> ALWQFNGMIKCKIPSSEPLLDFNNYGCYCGLGGSGTPVDDLDRCCQTHKNCYKQAKKLDSCKVLVDNPYTNNYSYSCSNNEITCSSENNACEAFICNCDRNAAICFSKVPYNKEHKNLDK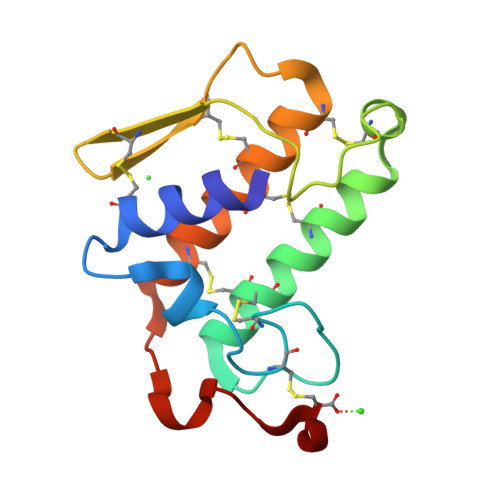KNC>[2x]AANDPFTIVHGNTGKCIKPVYGWIVADDCDETEDKLWKWVSQHRLFHLHSQKCLGLDITKSVNELRMFSCDSSAMLWWKCEHHSLYGAARYRLALKDGHGTAISNASDVWKKGGSEESLCDQPYHEIYTRDGNSYGRPCEFPFLIDGTWHHDC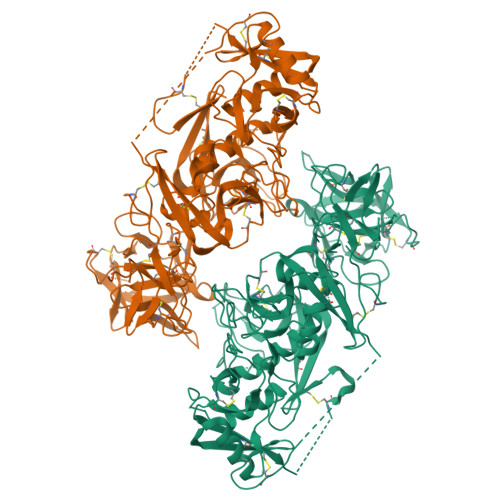ILDEDHSGPWCATTLNYEYDRKWGICLKPENGCEDNWEKNEQFGSCYQFNTQTALSWKEAYVSCQNQGADLLSINSAAELTYLKEKEGIAKIFWIGLNQLYSARGWEWSDHKPLNFLNWDPDRPSAPTIGGSSCARMDAESGLWQSFSCEAQLPYVCRKPLNNTVELTDVWTYSDTRCDAGWLPNNGFCYLLVNESNSWDKAHAKCKAFSSDLISIHSLADVEVVVTKLHNEDIKEEVWIGLKNINIPTLFQWSDGTEVTLTYWDENEPNVPYNKTPNCVSYLGELGQWKVQSCEEKLKYVCKRKGEKLNDASSDKMCPPDEGWKRHGETCYKIYEDEVPFGTNCNLTITSRFEQEYLNDLMKKYDKSLRKYFWTGLRDVDSCGEYNWATVGGRRRAVTFSNWNFLEPASPGGCVAMSTGKSVGKWEVKDCRSFKALSICKKMSHHHHHH> SVFAYESSVHSTNVLLSLNDQRKKDVLCDVTIFVEGQRFRAHRSVLAACSSYFHSRIVGQADGEL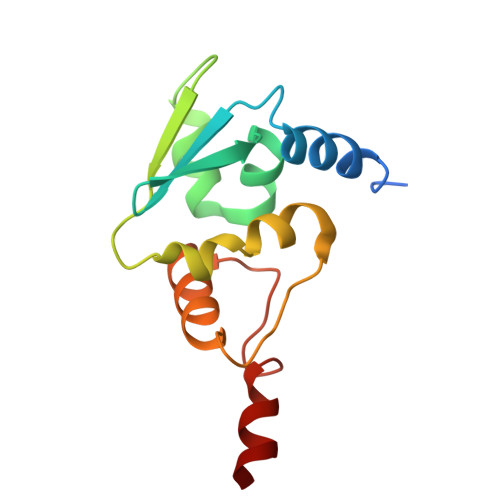NITLPEEVTVKGFEPLIQFAYTAKLILSKENVDEVCKCVEFLSVHNIEESCFQFLKFKFLD>[2x]GPLGSMAGPEGFQYRALYPFRRERPE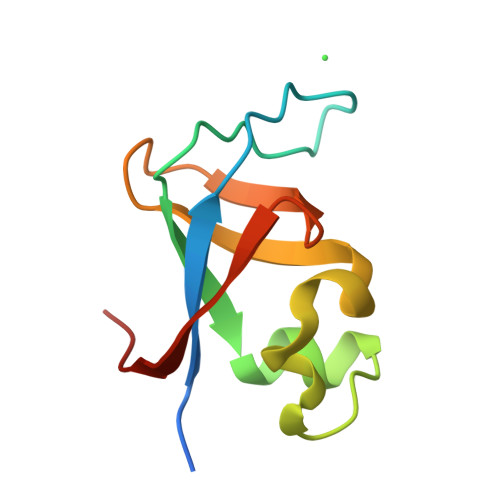DLELLPGDVLVVSRAALQALGVAEGGERCPQSVGWMPGLNERTRQRGDFPGTYVEFLGPVALAR>[4x]MRGLTVNFERINPMTNQTASTAKAMTAAEARAVADRAAAGFAGWSVLGPNARRAVLMKAAAALEARKDDFVQAMMAEIGATAGWAMFNLMLAASMIREAAALTTQIGGEVIPSDKPGCLALALREPVGVVLGIAPWNAPIILGVRAIAVPLACGNAVILKASEICPRTHGLIIESFAEAGFPEGVVNVVTNAPQDAGEVVGALIDHPAVKRINFTGSTGVGRIIAKRAAEHLKPCLLELGGKAPLVVLDDADLDEAAKAAAFGAFMNQGQICMSTERIIVVEAIAAEFTRRFAAKAQSMATGDPREGKTPLGAVVDRKTVDHVNTLIDDATAKGARIIAGGKGDSVLMSATVVDGVTAAMKLYRDESFGPIVGIIRAKDEADAVRLANDSEYGLAAAVFTRDTARGLRVARQIRSGICHINGPTVHDEAQMPFGGVGASGYGRFGGKAGIDQFTELRWITMETQPGHFPI

Gene-targeted assembly was used to mine a novel salicylaldehyde dehydrogenase from an Alpine soil metagenome. As a key intermediate in the breakdown of some aromatic PAHs, salicylaldehyde can be oxidized to salicylate by the activity of salicylaldehyde dehydrogenase (SALD; EC 1.2.1.65), which is an NAD(P)+-dependent enzyme. SALD belongs to the superfamily of NAD(P)+-dependent aldehyde dehydrogenases (ALDHs). Generally, the enzymes of this superfamily catalyse the oxidation of a broad range of aldehydes to their corresponding carboxylic acids, playing a major role in detoxification.

The crystals grew in the orthorhombic space group C2221, with unit-cell parameters a = 116.8, b = 121.7, c = 318.0 Å, and diffracted to 1.9 Å resolution. Polypeptide chains A and C formed the first dimer, while chains B and D formed the second homodimer. SALDAP adopts the standard conformation of the ALDH superfamily. The monomer shows that the enzyme is a classical aldehyde dehydrogenase showing the typical α/β aldehyde dehydrogenase superfamily organization with three domains: catalytic, NAD+-binding and bridging domains. The biological unit (dimer) of SALDAP is formed by the oligomerization of two monomers through the bridging domain. The oligomerization domain is typical of that found in class 3 ALDHs, with the C-terminal portion of the protein pointing away from a position that favours the interaction of a dimer–dimer interface (tetramer), thus only favouring the formation of a dimer. Although the EDs were good, protocatechuic acid (PCA) was chosen as the ligand bound to the active site for refinement as it fitted the ED better. A hydrogen bond between the para-hydroxyl group of the ligand and the Asp427 side chain is indicated as a black broken line in Fig. 3(a). Interestingly, the binding of a carboxylic acid in the active site of the aldehyde dehydro­genase indicates the potential for product inhibition of the enzyme during aldehyde oxidation; this also means that the enzyme may possess carboxylic acid reductase activity. Although an NAD+ molecule was not found in the cofactor-binding site, the potential residues implicated in the interaction with NAD+ adopted a fold quite similar to those observed in other NAD+-dependent ALDH complex structures.The KdpDE two-component system regulates potassium homeostasis and virulence in various bacterial species. The KdpD histidine kinases (HK) of this system contain a universal stress protein (USP) domain which binds to the second messenger cyclic-di-adenosine monophosphate (c-di-AMP) for regulating transcriptional output from this two-component system in Firmicutes such as Staphylococcus aureus. The KdpD HKs of this TCS are prototypical among membrane-anchored HKs that contain an N-terminal sensory cytoplasmic region (NTR) in addition to a canonical transmembrane domain and a cytoplasmic C-terminal region.

Here, we resolved a 2.3 Å crystal structure of the S. aureus KdpD-USP domain (USPSa) complexed with c-di-AMP. A sheet of five β-strands (β1-β5) in the structure is sandwiched between two layers of α-helices, with each layer containing two α-helices (α1-α2 and α3-α4). The c-di-AMP binding region in the USPSa was found to involve β1, α1, the β1-α1 loop, β2, the β2-α2 loop, β4, and the β4-α4 loop. One of the two AMP moieties of the c-di-AMP in the USPSa:c-di-AMP structure occupies a pocket similar to the ATP-binding pocket in the USPFG subfamily of proteins, which we refer to as the “inner AMP” (see the Experimental procedures section). The other AMP moiety of c-di-AMP in the USPSa:c-di-AMP structure projects outward from the “ATP-binding pocket”, and we refer to it as the “outer AMP”. The c-di-AMP in the USPSa:c-di-AMP structure adopts a V-shaped conformation with a C6-C6 distance of 8.3 Å. Similar to USPATP proteins, the side chains of the first two β2 stretch residues in USPSa (Ile270 and Tyr271) are able to form hydrophobic contacts with the inner adenine ring of c-di-AMP, and the main chain carboxyl and amino groups of the third residue (Ile272) form hydrogen bonds with adenine N6 and N1, respectively. Tyr281 interacts with both the inner and the outer AMPs in c-di-AMP by (i) forming antiparallel sandwich-type π-stacking interactions with its terminal hydroxyl facing N7 and N9 of the outer adenine ring and by (ii) forming a water-mediated hydrogen bond with the inner phosphoryl oxygen. While the absence of a Walker A motif in the β4-α4 loop of USPSa could alone accomplish the ATP-binding loss, this loop was found to adopt a conformation that is structurally distinct from its conformation in standalone USPFG proteins. Interestingly, USPSa seems to utilize both the α1-binding mode and the α4-binding mode to interact with the inner and outer AMP moieties in c-di-AMP.

> TLRTVADLMSDKEKVRHNHKTSLKPHIAVAISGSIYNEAVIKEAFHIAQKEHAKFTAIYIDVFEKSRQYKDSQKQVHQHLMLAKSLGAKVKVVYSQTVALGLDEWCKNQDVTKLIIGQHIRNKRRDFFNKPLIDHLMSFEHSYKIEIVPIKQ> GSMRNELEEMQRRADQ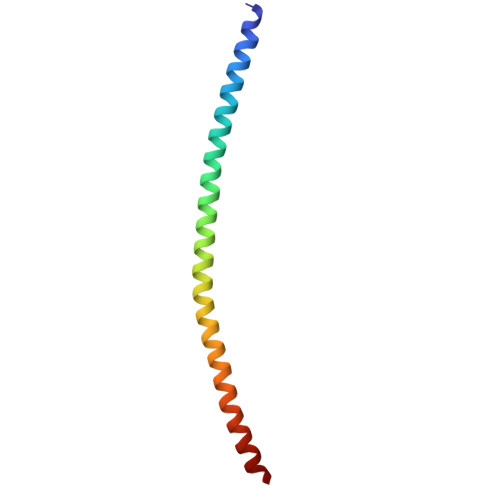LADESLESTRRMLQLVEESKDAGIRTLVMLDEQGEQLDRVEEGMNHINQDMKEAEKNLKDLGK> MLEETEAALLARVRELFGATLRQVEPLTGTWTNEDVHRLFLAPPSVFLAWMGCGEGRTRREVESRWAFFVV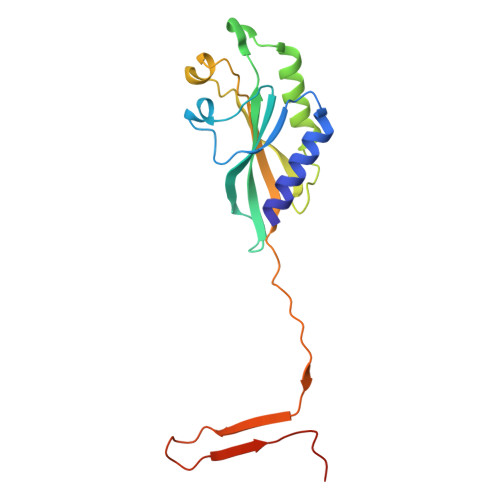AELLNGEPVNRPGIYQIVERLIAGVNGQTFGPTTGMRLTQVRNLCDDNRINAGVVLYGVLFSGTTPLPSVVDLDSLDDYERHWQTWKFPDETPEFAAHINVNQEKDHDAEN> QVTVQSSPNFTQHVREQSLVTDQLSRRLIRTYQLYSRTSG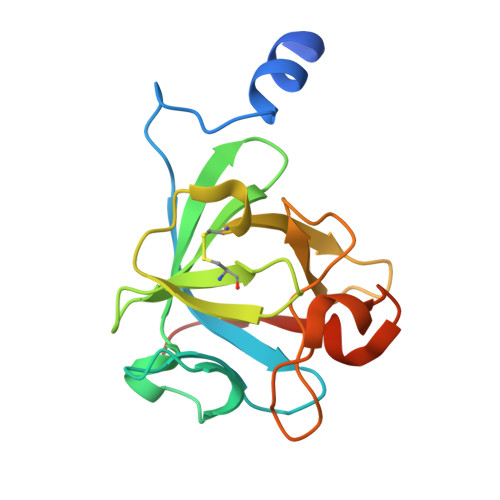KHVQVLANKRINAMAEDGDPFAKLIVETDTFGSRVRVRGAETGLYICMNKKGKLIAKSNGKGKDCVFTEIVLENNYTALQNAKYEGWYMAFTRKGRPRKGSKTRQHQREVHFMKRLPRGHHTTE>MGSSHHHHHHSSGENLYFQGSHMVGEKEYKAWEKKLRANEKELVKEYTANAKPFNTYLRANEGKLGFKPEIDKKILKLDEALKKSKLSETVQVYRGDDTSIFGKEFQNSIYQGNKVNRELFRKLRDEYQGKIRTEYGYLSTSIV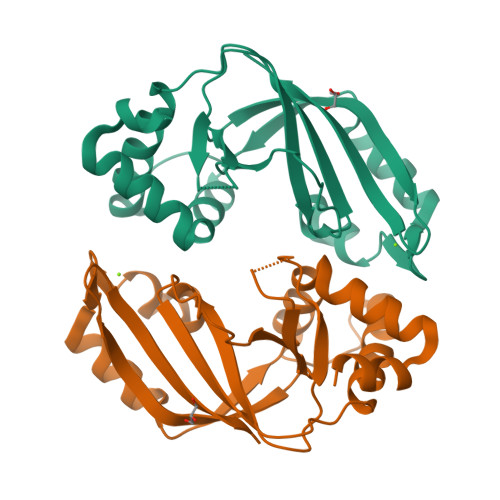SNQQFAMRPVLTTLKVPKGAHAGYVDKISQYKGQYELLLPRNTKYKIDKMYIIVNKGSETIKIEATVQP[2x]DNA double-strand breaks that initiate meiotic recombination are formed by the topoisomerase-relative enzyme Spo11, supported by conserved auxiliary factors. We report cryo-electron microscopy structures at up to 3.3-Å resolution of DNA-bound core complexes of Saccharomyces cerevisiae Spo11 with Rec102, Rec104 and Ski8. The core complex is monomeric (1:1:1:1 stoichiometry) and adopts a V shape with Spo11 at the base contacting the three other subunits. Spo11 is a central hub making extensive protein–protein and protein–DNA contacts.

We also solved the structure of the core complex bound to a double-hairpin substrate with a single-stranded DNA (ssDNA) gap at 3.3-Å resolution. The preference for binding to bent DNA14 motivated these experiments, on the premise that the ssDNA region would provide the flexibility needed to assemble dimeric complexes that resemble the pre-DSB state. However, the majority of particles again had just a single core complex. We can trace the duplex of one hairpin plus the first nucleotide of the ssDNA (A39) including its 5′-phosphate. The bound hairpin is the one with a free 3′-OH and ssDNA extending from the 5′ end, which is structurally analogous to the single hairpin initially used. Weak density in the unsharpened map spanned the single-stranded nucleotides T38-T37-A36 and a portion of the second hairpin, with the two duplex segments aligned at a relative angle of 130°. The structures with hairpin DNA and gapped DNA superpose well (root-mean-square deviation (r.m.s.d.) = 1.23 Å); hence, the following sections focus on the higher-resolution gapped-DNA structure. Patch 1 anchors overhang nucleotide A39 and its adjacent duplex in the pocket between the Spo11 WH and Toprim domains. R131 on the second α-helix of the WH domain forms a hydrogen bond with the 5′-phosphate of G40, which is the bridging phosphate between the first base of the duplex (G40) and the beginning of the 5′ overhang (A39). Moreover, the contacts of R131 and Q144 with the 5′-phosphate at the beginning of the duplex and of E233 with the 3′-hydroxyl explain the strong selectivity for a free 3′-OH end and 5′ ssDNA overhang.

> MALEGLRKKYKTRQELVKALTPKRRSIHLNSNGHSNGTPCSNADVLAHIKHFLSLAANSLEQHQQPISIVFQNKKKKGDTNSPDIHTTLDFPLNGPHLSTHQFKLKRCAILLNLLKVVMEKLPLGKNTTVRDIFYSNVELFQRQANVVQWLDVIRFNFKLSPRKSLNIIPAQKGLVYSPFPIDIYDNILTCENEPKMQKQTIFSGKPCLIPFFQDDAVIKLGTTSMCNIVIVEKEAVFTKLVNNYHKLSTNTMLITGKGFPDFLTRLFLKKLEQYCSNLISDCSIFTDADPYGISIALNYTHSNERNAYICTMANYKGIRITQVLAQNNEVHNKSIQLLSLNQRDYSLAKNLIASLTANSWDIATSPLKNVVIECQREIFFQKKAEMNEIDAGIFKYKSRHHHHHHHHHHGDYKDDDDKDYKDDDDKDYKDDDDK;> MARDITFLTVFLESCGAVNNDEAGKLLSAWTSTVRIEGPESTDSNSLYIPLLPPGMLKIKLNFKMNDRLVTEEQELFTKLREIVGSSIRFWEEQLFYQVQDVSTIENHVILSLKCTILTDAQISTFISKPRELHTHAKGYPEIYYLSELSTTVNFFSKEGNYVEISQVIPHFNEYFSSLIVSQLEFEYPMVFSMISRLRLKWQQSSLAPISYALTSNSVLLPIMLNMIAQDKSSTTAYQILCRRRGPPIQNFQIFSLPAVTYNK;> MSKVFIATANAGKAHDADIFSVSACNSFTVSCSGDGYLKVWDNKLLDNENPKDKSYSHFVHKSGLHHVDVLQTIERDAFELCLVATTSFSGDLLFYRITREDETKKVIFEKLDLLDSDMKKHSFWALKWGASNDRLLSHRLVATDVKGTTYIWKFHPFADESNSLTLNWSPTLELQGTVESPMTPSQFATSVDISERGLIATGFNNGTVQISELSTLRPLYNFESQHSMINNSNSIRSVKFSPQGSLLAIAHDSNSFGCITLYETEFGERIGSLSVPTHSSQASLGEFAHSSWVMSLSFNDSGETLCSAGWDGKLRFWDVKTKERITTLNMHCDDIEIEEDILAVDEHGDSLAEPGVFDVKFLKKGWRSGMGADLNESLCCVCLDRSIRWFREAGGK;> MSIEEEDTNKITCTQDFLHQYFVTERVSIQFGLNNKTVKRINKDEFDKAVNCIMSWTNYPKPGLKRTASTYLLSNSFKKSATVSLPFILGDPVCMPKRVESNNNDTCLLYSDTLYDDPLIQRNDQAGDEIEDEFSFTLLRSEVNEIRPISSSSTAQILQSDYSALMYERQASNGSIFQFSSP>MPDMANVESFDLDHTKVKAPYVRLAGVKTTPKGDQISKYDLRFLQPNQGAIDPAAIHTLEHLLAGYMRDHLEGVVDVSPMGCRTGMYMAVIGEPDEQGVMKAFEAALKDTAGHDQPIPGVSELECGNYRDHDLAAARQHARDVLDQGLKVQETILLERGS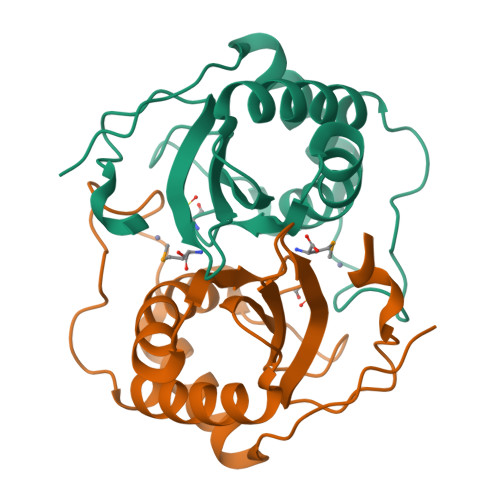HHHHHH[2x]> MDALDASKLLDEELYSRQLYVLGSPAMQRIQGARVLVSGLQGLGAEVAKNLVLMGVGSLTLHDPHPTCWSDLAAQFLLSEQDLERSRAEASQELLAQLNRAVQVVVHTGDITEDLLLDFQVVVLTAAKLEEQLKVGTLCHKHGVCFLAADTRGLVGQLFCDFGEDFTVQDPTEAEPLTAAIQHISQGSPGILTLRKGANTHYFRDGDLVTFSGIEGMVELNDCDPRSIHVREDGSLEIGDTTTFSRYLRGGAITEVKRPKTVRHKSLDTALLQPHVVAQSSQEVHHAHCLHQAFCALHKFQHLHGRPPQPWDPVDAETVVGLARDLEPLKRTEEEPLEEPLDEALVRTVALSSAGVLSPMVAMLGAVAAQEVLKAISRKFMPLDQWLYFDALDCLPEDGELLPSPEDCALRGSRYDGQIAVFGAGFQEKLRRQHYLLVGAGAIGCELLKVFALVGLGAGNSGGLTVVDMDHIERSNLSRQFLFRSQDVGRPKAEVAAAAARGLNPDLQVIPLTYPLDPTTEHIYGDNFFSRVDGVAAALDSFQARRYVAARCTHYLKPLLEAGTSGTWGSATVFMPHVTEAYRAPASAAASEDAPYPVCTVRYFPSTAEHTLQWARHEFEELFRLSAETINHHQQAHTSLADMDEPQTLTLLKPVLGVLRVRPQNWQDCVAWALGHWKLCFHYGIKQLLRHFPPNKVLEDGTPFWSGPKQCPQPLEFDTNQDTHLLYVLAAANLYAQMHGLPGSQDWTALRELLKLLPQPDPQQMAPIFASNLELASASAEFGPEQQKELNKALEVWSVGPPLKPLMFEKDDDSNFHVDFVVAAASLRCQNYGIPPVNRAQSKRIVGQIIPAIATTTAAVAGLLGLELYKVVSGPRPRSAFRHSYLHLAENYLIRYMPFAPAIQTFHHLKWTSWDRLKVPAGQPERTLESLLAHLQEQHGLRVRILLHGSALLYAAGWSPEKQAQHLPLRVTELVQQLTGQAPAPGQRVLVLELSCEGDDEDTAFPPLHYEL;> MGWDLTVKMLAGNEFQVSLSSSMSVSELKAQITQKIGVHAFQQRLAVHPSGVALQDRVPLASQGLGPGSTVLLVVDKSDEPLSILVRNNKGRSSTYEVRLTQTVAHLKQQVSGLEGVQDDLFWLTFEGKPLEDQLPLGEYGLKPLSTVFMNLRLRGG;> MASMRVVKELEDLQKKPPPYLRNLSSDDANVLVWHALLLPDQPPYHLKAFNLRISFPPEYPFKPPMIKFTTKIYHPNVDENGQICLPIISSENWKPSTKTSQVLEALNVLVNRPNIREPKRMDLADLLTQNPELFRKNAEEFTLRFGVDRPS

ISG15 is a ubiquitin-like protein that is activated by an E1 enzyme (Uba7) and transferred to a cognate E2 enzyme (UBE2L6) to form a UBE2L6-ISG15 intermediate that functions with E3 ligases that catalyze conjugation of ISG15 to target proteins. E1 occupies the apex of the Ub/Ubl conjugation cascade where it performs two main functions: (1) specific activation of Ub/Ubl in a two-step process that results in the formation of a thioester bond between Ub/Ubl and an E1 catalytic cysteine (adenylation and thioester bond formation) and (2) recruitment of cognate E2 enzymes followed by transfer of Ub/Ubl to an E2 catalytic cysteine (thioester transfer). While Uba1 (E1) is specific to Ub activation, ISG15 is exclusively activated by Uba7 (E1) and specifically transferred to the E2 enzyme UBE2L6. Here, we present cryo-EM structures of human Uba7 in complex with UBE2L6, ISG15 adenylate, and ISG15 thioester intermediate in a conformational state that is poised for catalysis of Uba7-UBE2L6-ISG15 thioester transfer.

Previous studies in the Ub system have shown that although the single-loaded E1-E2-Ub(t) complex is capable of catalyzing thioester transfer, that double-loaded E1 is significantly more efficient at E2 recruitment and catalysis. Although modestly ordered, the ISG15(t) projects away from the surface of UBE2L6 towards the ‘back’ of the complex where it sits atop the AAD, sandwiched between the UFD and SCCH domain. This result was somewhat unexpected based on a previous structure of Uba1/CDC34-Ub(t) in which two distinct ‘open’ and ‘closed’ conformations of Ub(t) were observed that both reside on the front side of the complex. To validate that the density on the backside of the Uba7-UBE2L6-ISG15(t)/ISG15(a) complex indeed belongs to ISG15(t), we solved the cryo-EM structure single-loaded Uba7-UBE2L6/ISG15(a) complex lacking ISG15(t), with a nominal resolution of 3.24 Å (masked at 0.143 FSC). Analysis of the cryo-EM density reveals no density in the back of the complex that corresponds to the density present in the double-loaded Uba7-UBE2L6-ISG15(t)/ISG15(a) complex structure we ascribe to the ISG15(t) CTD. With respect to the ISG15(a) NTD/UFD interaction, these contacts may serve as a sensor for the presence of ISG15(a) in double-loaded Uba7/UBE2L6/ISG15 complex and provide an additional mechanism as to why double-loaded complex is more efficient at thioester transfer compared to the single-loaded counterpart.> MRVLILGVNGFIGNHLTERLLREDHYEVYGLDIGSDAISRFLNHPHFHFVEGDISIHSEWIEYHVKKCDVVLPLVAIATPIEYTRNPLRVFELDFEENLRIIRYCVKYRKRIIFPSTSEVYGMCSDKYF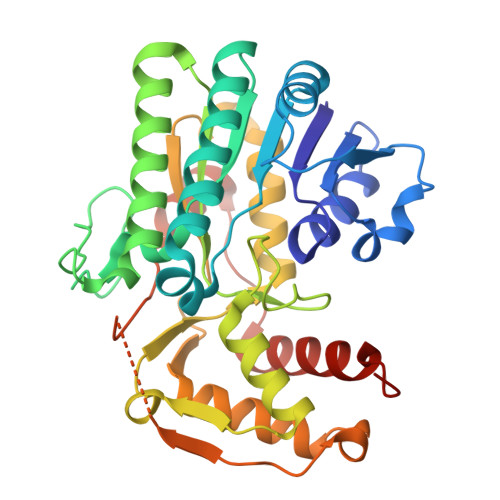DEDHSNLIVGPVNKPRWIYSVSKQLLDRVIWAYGEKEGLQFTLFRPFNWMGPRLDNLNAARIGSSRAITQLILNLVEGSPIKLIDGGKQKRCFTDIRDGIEALYRIIENAGNRCDGEIINIGNPENEASIEELGEMLLASFEKHPLRHHFPPFAGFRVVESSSYYGKGYQDVEHRKPSIRNAHRCLDWEPKIDMQETIDETLDFFLRTVDLTDKPS> TLSILVAHDLQRVIGFENQLPWHLPNDLKHVKKLSTGHTLVMGRKTFESIGKPLPNRRNVVL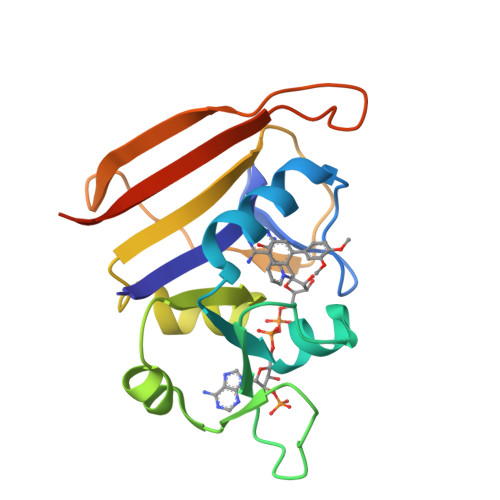TSDTSFNVEGVDVIHSIEDIYQLPGHVFIFGGQTLFEEMIDKVDDMYITVIEGKFRGDTFFPPYTFEDWEVASSVEGKLDEKNTIPHTFLHLIRKKLEHHHHHH>[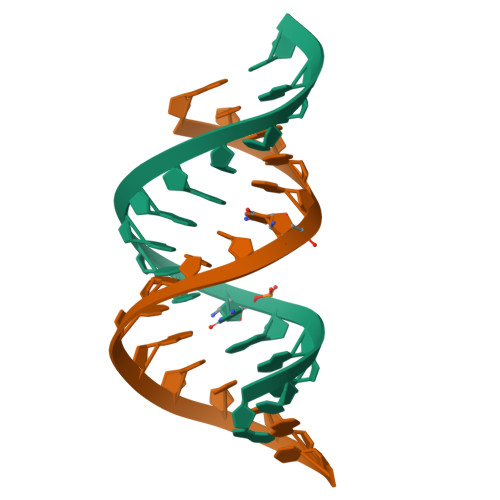3x]GCAGACUUAAAUCUGC GUANOSINE-5'-PHOSPHATE-2',3'-CYCLIC PHOSPHATE | C10 H13 N5 O10 P2 | 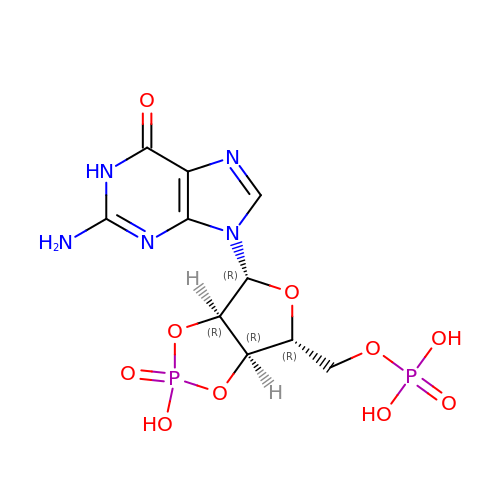ZBMMALUAVDLKSL-UUOKFMHZSA-N>MTPESVMMMGTEAMKVALALAAPLLLVALITGLIISILQAATQINEMTLSFIPKIVAVFIAIIVAGPWMLNLLLDYVRTLFSNLPYIIG[4x];> MIQVTSEQWLYWLHLYFWPLLRVLALISTAPILSERAIPKRVKLGLGIMITLVIAPSLPANDTPLFSIAALWLAMQQILIGIALGFTMQFAFAAVRTAGEFIGLQMGLSFATFVDPGSHLNMPVLARIMDMLAMLLFLTFNGHLWLISLLVDTFHTLPIGSNPVNSNAFMALARAGGLIFLNGLMLALPVITLLLTLNLALGLLNRMAPQLSIFVIGFPLTLTVGIMLMAALMPLIAPFCEHLFSEIFNLLADIVSEMPINNNP;>MRRLLFLSLAGLWLFSPAAAAQLPGLISQPLAGGGQSWSLSVQTLVFITSLTFLPAILLMMTSFTRIIIVFGLLRNALGTPSAPPNQVLLGLALFLTFFIMSPVIDKIYVDAYQPFSEQKISMQEALDKGAQPLRAFMLRQTREADLALFARLANSGPLQGPEAVPMRILLPAYVTSELKTAFQIGFTIFIPFLIIDLVIASVLMALGMMMVPPATIALPFKLMLFVLVDGWQLLMGSLAQSFYS[5x];>[6x]MAAIQGIEGVISQLQATAMAARGQDTHSQSTVSFAGQLHAALDRISDRQAAARVQAEKFTLGEPGIALNDVMADMQKASVSMQMGIQVRNKLVAAYQEVMSMQV;>MLDRLDAALRFQQEALNLRAQRQEILAANIANADTPGYQARDIDFASELKKVMVRGREETGGVALTLTSSHHIPAQAVSSPAVDLLYRVPDQPSLDGNTVDMDRERTQFADNSLKYQMGLTVLGSQLKGMMNVLQGGN[5x];>[6x]MALLNIFDIAGSALAAQSKRLNVAASNLANADSVTGPDGQPYRAKQVVFQVDAAPGQATGGVKVASVIESQAPEKLVYEPGNPLADANGYVKMPNVDVVGEMVNTMSASRSYQANIEVLNTVKSMMLKTLTLGQ;>MSATASTATQPKPLEWLNRLRANPRIPLIVAGSAAVAIVVAMVLWAKTPDYRTLFSNLSDQDGGAIVAQLTQMNIPYRFANGSGAIEVPADKVHELRLRLAQQGLPKGGAVGFELLDQEKFGISQFSEQVNYQRALEGELARTIETLGPVKSARVHLAMPKPSLFVREQKSPSASVTVTLEPGRALDEGQISAVVHLVSSAVAGLPPGNVTLVDQSGHLLTQSNTSGRDLNDAQLKFANDVESRIQRRIEAILSPIVGNGNVHAQVTAQLDFANKEQTEEHYSPNGDASKATLRSRQLNISEQVGAGYPGGVPGALSNQPAPPNEAPIATPPTNQQNAQNTPQTSTSTNSNSAGPRSTQRNETSNYEVDRTIRHTKMNVGDIERLSVAVVVNYKTLADGKPLPLTADQMKQIEDLTREAMGFSDKRGDTLNVVNSPFSAVDNTGGELPFWQQQSFIDQLLAAGRWLLVLVVAWILWRKAVRPQLTRRVEEAKAAQEQAQVRQETEEAVEVRLSKDEQLQQRRANQRLGAEVMSQRIREMSDNDPRVVALVIRQWMSNDHE[11x];>[5x]MDHAIYTAMGAASQTLNQQAVTASNLANASTPGFRAQLNALRAVPVDGLSLATRTLVTASTPGADMTPGQLDYTSRPLDVALQQDGWLVVQAADGAEGYTRNGNIQVGPTGQLTIQGHPVIGEGGPITVPEGSEITIAA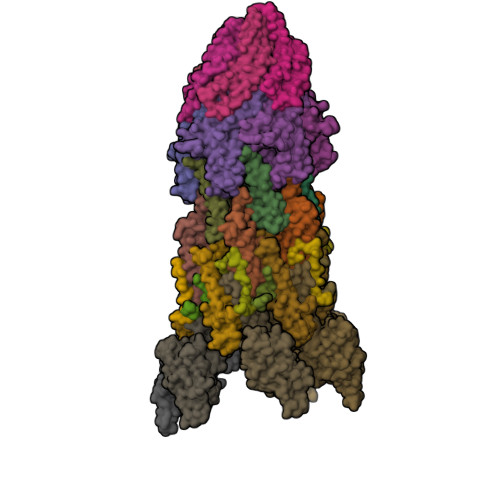DGTISALNPGDPPNTVAPVGRLKLVKAEGNEVQRSDDGLFRLTAEAQAERGAVLAADPSIRIMSGVLEGSNVKPVEAMTDMIANARRFEMQMKVITSVDENEGRANQLLSMS> SPVAPACDPRLLNKLLRDSHLLHSRLSQCPDVDPLSIPVLLPAVDFSLGE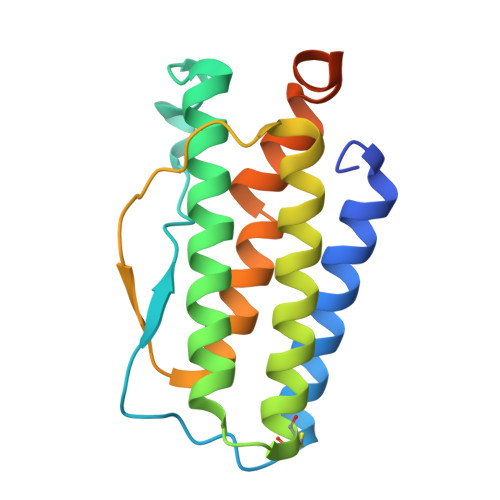WKTQTEQSKAQDILGAVSLLLEGVMAARGQLEPSCLSSLLGQLSGQVRLLLGALQGLLGTQLPLQGRTTAHKDPNALFLSLQQLLRGKVRFLLLVEGPTLCVRRTLPTTAVPSENLYFQG N-[2-(acetylamino)ethyl]-N~3~-[(2R)-2-hydroxy-3,3-dimethyl-4-(phosphonooxy)butanoyl]-beta-alaninamide 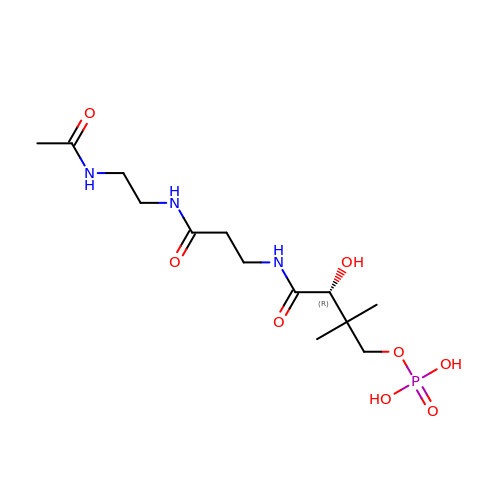| C13 H26 N3 O8 P | GTANJSAWPNEGPZ-NSHDSACASA-N>QANLMRLKSDLFNRSPMYPGPTKDDPLTVTLGFTLQDIVKVDSSTNEVDLVYYEQQRWKLNSLMWDPNEYGNITDFRTSAADIWTPDITAYSSTRPVQVLSPQIAVVTHDGSVMFIPAQRLSFMCDPTGVDSEEGVTCAVKFGSWVYSGFEIDLKTDTDQVDLSSYYASSKYEI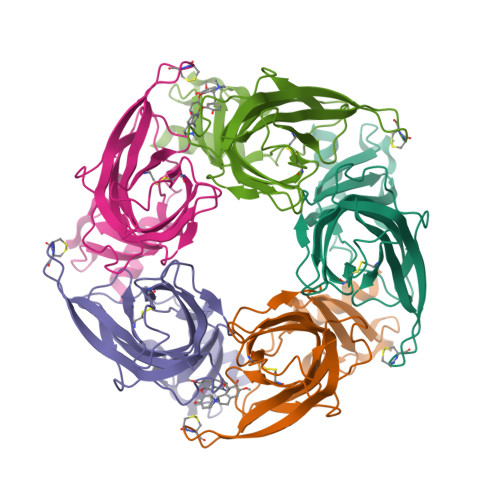LSATQTRQVQHYSCCPEPYIDVNLVVKFRERRAGNGFFRNLFD[10x]> GPLGSMSAAIAKPSAKPSAHVDPKSAPLKEIP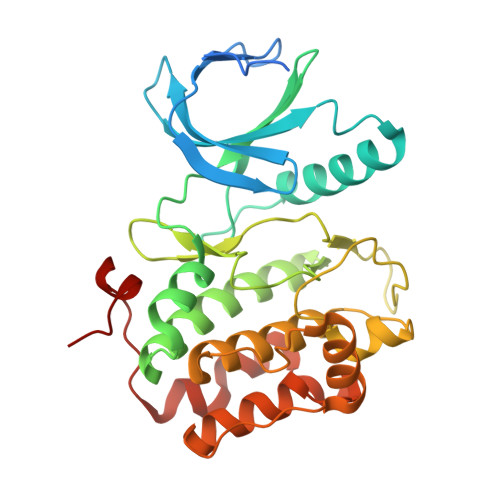DVLVDPRTMKRYMRGRFLGKGGFAKCYEITDMDTKEVFAGKVVPKSMLLKPHQKEKMSTEIAIHKSLDNPHVVGFHGFFEDDDFVYVVLEICRRRSLLELHKRRKAVTEPEARYFMRQTIQGVQYLHNNRVIHRDLKLGNLFLNDDMDVKIGDFGLATKIEFDGERKKTLCGTPNYIAPEVLCKKGHSFEVDIWSLGCILYTLLVGKPPFETSCLKETYIRIKKNEYSVPRHINPVASALIRRMLHADPTLRPSVAELLTDEFFTSGYAPMRLPTSCLTVPPRFS>MNTTPVHALTDIDGGIAVDPAPRLAGPPVFGGPGNDAFDLAPVRSTGREMLRFDFPGVSIGAAHYEEGPTGATVIHIPAGARTAVDARGGAVGLSGGYDFNHAICLAGGAGYGLEAGAGVSKALLERLEHRTGFAELQLVSSAVIYDFSARSTAVYPDKALGRAALEFAVPGEFPQGRAGAGMSASAGKVDWDRTEITGQGAAFRRLGDVRILAVVVPNPVGVIVDRAGT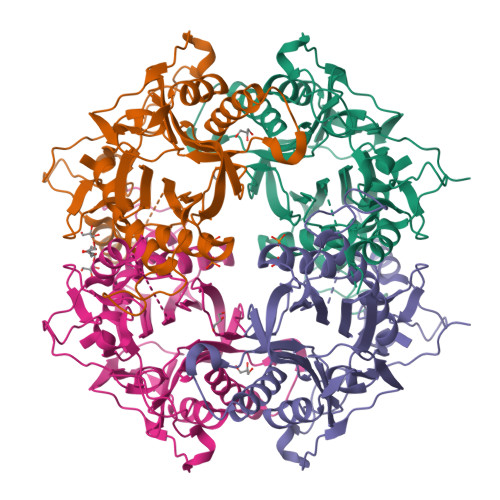VVRGNYDAQTGVRRHPVFDYQEAFAEQVPPVTEAGNTTISAIVTNVRMSPVELNQFAKQVHSSMHRGIQPFHTDMDGDTLFAVTTDEIDLPTTPGSSRGRLSVNATALGAIASEVMWDAVLEAGK[2x]2'-deoxy-5-fluorocytidine 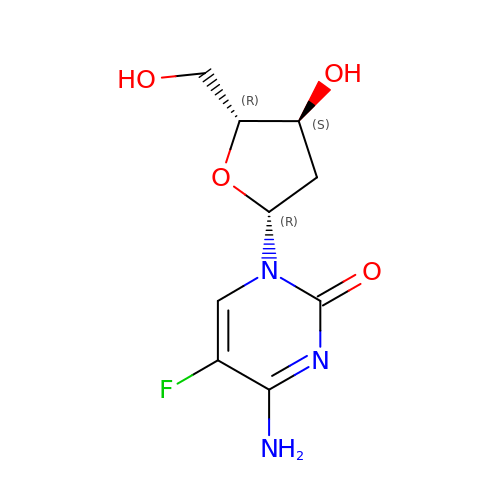| C9 H12 F N3 O4 | IDYKCXHJJGMAEV-RRKCRQDMSA-N>MQLFDLSLEELKKYKPKKTARPDFADFWKKSLEELRQVEAEPTLESYDYPVKGVKVYRLTYQSFGHSKIEGFYAVPDQTGPHPALVRFHGYNASYDDGIHDIVNWALHGYATFGMLVRGQGGSEDTSVTPGGHALGWMTKGILSKDTYYYRGVYLDAVRALEVIQSFPEVDEHRIGVIGGSQGGALAIAAAALSDIPKVVVADYP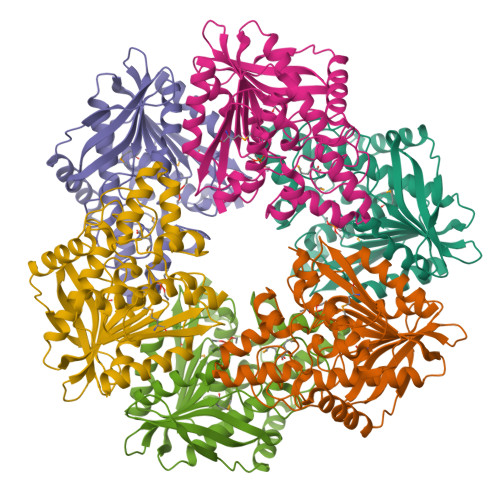YLSNFERAVDVALEQPYLEINSYFRRNSDPEVEEKAFETLSYFDLINLAGWVKQPTLMAIGLIDQVTPPSTVFAAYNHLETDKELKVYRYFGHEFIPAFQTEKLSFLQKHLLLST[6x]>SKPQPIAAANWKSGSPDSLSELIDLFNSTSINHDVQCVVASTFVHLAMTKERLSHPKFVIAAQNAGNADALASLKDFGVNWIVLGHSERRWYYGETNEIVADKVAAAVASGFMVIACIGETLQERESGR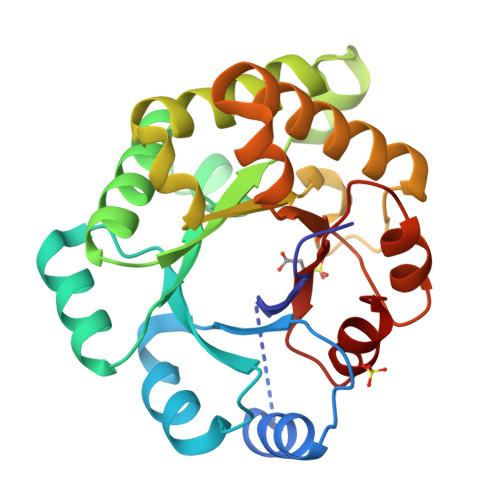TAVVVLTQIAAIAKKLKKADWAKVVIAYEPVWAIGTGKVATPQQAQEAHALIRSWVSSKIGADVAGELRILYGGSVNGKNARTLYQQRDVNGFLAGLKPEFVDIIKATQ[2x]One example where the lack of enzyme regioselectivity limits potential commercial productivity is the engineered biosynthesis of the flavor and fragrance agent vanillin 2 a.3 Catechol‐O‐methyltransferase (COMT) has been used to methylate 3,4‐dihydroxybenzaldehyde (DHBAL, 1 a) and 3,4‐dihydroxybenzoic acid (DHBA, 1 b) in engineered strains of Escherichia coli and fission yeast for the production of vanillin 2 a from glucose. However, the lack of regioselectivity of COMT results in a mixture of 2 a and the undesired para‐methylated isovanillin 3 a, which are difficult to separate. Structural and mechanistic information suggest that the regioselectivity of COMT can be attributed to the concerted action of a “hydrophobic wall” found in the active site of the enzyme, and the substrate properties. The orientation of the R group in the active site determines whether the meta‐ or para‐hydroxy group is methylated.

Gel filtration chromatography showed two different oligomeric states for COMT. The WT monomer showed significantly lower re values of +31 % (1 a), +48 % (1 b), and +33 % (1 d) compared to +84 % (1 a), +59 % (1 b), +87 % (1 d) for the dimer. Unlike with monomeric WT COMT, the β7 strand exchange between the two subunits that occurs in the dimer maintains the overall Rossman fold tertiary structure; however, E199 and Y200 lie on the β6–β7 interconnecting loop, which is pulled out of the active site as a result of domain swapping, thus leading to loss of the E199–substrate interaction. The X‐ray crystal structures of dimeric Y200L and WT COMT revealed that a key residue (E199) had been flipped out of the active site. We rationalize that in the WT monomeric enzyme, E199 can form a hydrogen bond with the aldehyde group of 1 a, thereby leading to some para‐methylation, whereas in dimeric Y200L and WT COMT the absence of E199 from the active site results in the aldehyde group orientating towards the solvent, thereby leading to meta‐methylation. Since monomeric Y200L is as regioselective as the dimeric forms (ca. +90 % re), we suggest, based on the structural data for the Y200L and WT dimers and the regioselectivity assay data for both oligomeric forms, that loss of para‐methylation is largely due to movement of E199 out of the active site, as a consequence either of mutagenesis (Y200L) or protein dimerization and domain swapping (WT). The physiologically relevant form of COMT in vivo may be the dimer, since mainly meta‐methylated catecholamine metabolites are found in urine and liver samples. However, another explanation is that the hexa‐His tag that we introduced at the C‐terminus may have contributed to domain swapping and dimerization.

> DTKEQRILRYVQQNAKPGDPQSVLEAIDTYCTQKEWAMNVGDAKGQIMDAVIREYSPSLVLELGAYCGYSAVRMARLLQPGARLLTMEMNPDYAAITQQMLNFAGLQDKVTILNGASQDLIPQLKKKYDVDTLDMVFLDHWKDRYLPDTLLLEKCGLLRKGTVLLADNVIVPGTPDFLAYVRGSSSFECTHYSSYLEYMKVVDGLEKAIYQGP2-[(2-carboxyphenyl)amino]-5-methylbenzoic acid | C15 H13 N O4 | 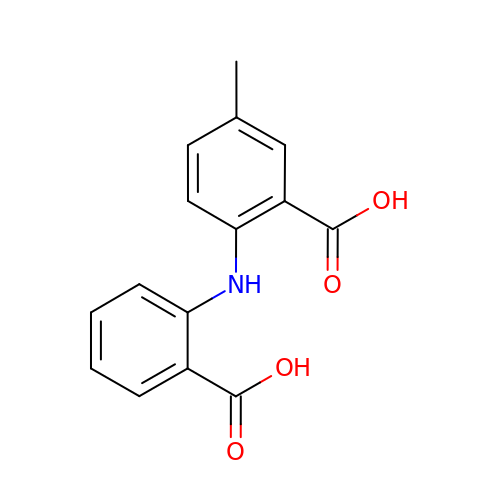KLVTUYAKQNFRLK-UHFFFAOYSA-N>[2x]SMLREDESACLQAAEEMPQTTLGCPATWDGLLCWPTAGSG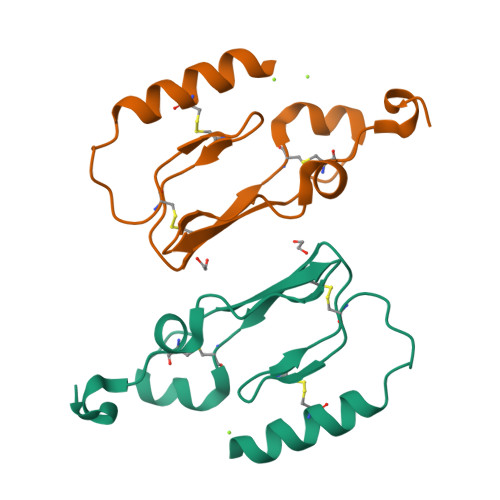EWVTLPCPDFFSHFSSESGAVKRDCTITGWSEPFPPYPVACPVPLELLAEEE>MKTLVHVASVEKGRSYEDFQKVYNAIALKLREDDEYDNYIGYGPVLVRLAWHTSGTWDKHDNTGGSYGGTYRFKK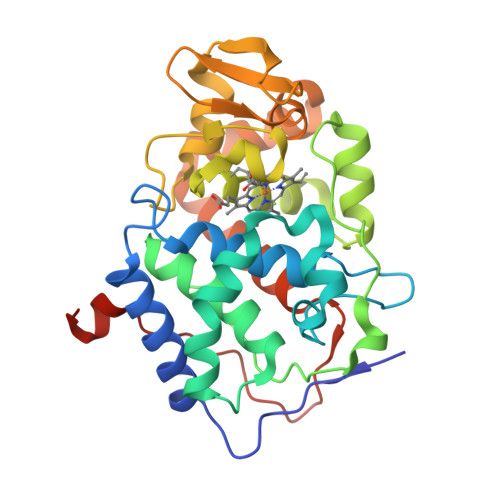EFNDPSNAGLQNGFKFLEPIHKEFPWISSGDLFSLGGVTAVQEMQGPKIPWRCGRVDTPEDTTPDNGRLPDADKDADYVRTFFQRLNMNDREVVALMGAHALGKTHLKNSGYEGPWGAANNVFTNEFYLNLLNEDWKLEKNDANNEQWDSKSGYMMLPTDYSLIQDPKYLSIVKEYANDQDKFFKDFSKAFEKLLENGITFPKDAPSPFIFKTLEEQGLHHHHHH[2x]> PLPTPVGMEIMPPQPPLPPDSSSQDCDPTASLRPFATKAEADAAVADIRARGRLIVGLDIGSNLFSFRDPITGEITGFDVDIAGEVARDIFGVPSHVEYRILSAAERVTALQKSQVDIVVKTMSITCERRKLVNFSTVYLDANQRILAPRDSPITKVSDLSGKRVCVARGTTSLRRIREIAPPPVIVSVVNWADCLVALQQREIDAVSTDDTILAGLVEEDPYLHIVGPDMADQPYGVGINLDNTGLVRFVNGTLERIRNDGTWNTLYRKWLTVLGPAPAPPTPRYVD

The conserved aspartate-specific solute-binding protein (SBP) GlnH links extracellular amino acid concentration to PknG activity via the periplasmic transmembrane protein GlnX, thereby controlling glutamate metabolism in Mycobacterium spp. GlnH belongs to the solute-binding protein family, specifically the polar amino acid binding family, which bind to arginine, cysteine, histidine, glutamine, glutamate, and aspartate. The fold of GlnH is related to bacterial solute-binding proteins from ATP transporters and to the sensor domains of glutamate receptors: two lobes close around the Asp ligand in a Venus flytrap-like arrangement. We propose that the amino acid concentration in the periplasm is sensed by GlnH and that protein-protein interaction allows transmission of this information across the membrane via GlnX to activate PknG.

To determine the structural basis of discrimination between higher- and lower-affinity ligands, GlnH was crystallized in the presence of Glu and Asn. Overall, the structures with different ligands bound were similar (Fig. 7A; root mean square deviation [RMSD] = 0.199 Å over 1,727 main-chain atoms). The greatest difference is in loops 99 to 103 and 109 to 113 (DIGSN and DPITG, respectively), which are displaced 2 Å in the Glu- or Asn-bound structures compared to the Asp-bound structure. The conformations of the ligand binding site and positioning of the ligands are similar. Contacts between GlnH and Glu are the same as those between GlnH and Asp, with the liganded Glu adopting a bent conformation such that the side-chain carboxyl group occupies the equivalent position to the side chain of ligand Asp in the GlnH-Asp complex. Glutamate and aspartate were identified as the stimuli that lead to rapid phosphorylation of GarA. Our structures of liganded GlnH represent “closed” conformations. Sequence alignment of GlnH homologues that are also genetically linked to PknG shows that within the order Actinomycetales (which includes important human and animal pathogens like Mycobacterium leprae and Rhodococcus equi), conservation of the residues that contact the R group of the Asp/Glu ligand predicts that these proteins are also likely to be specific for Asp and Glu.>[2x]MAHHHHHHVDDDDKMNSDDNADGLIFSPLPQNKNTVVRHYSNEQEMPNLSQMAQRTIDFPTQIVRVSGNLTGLELSCDDVENEIDQVFSKKISPNLFTYNTYVSCGYDVNDPEQHATNFSIQSYFDPLTDNAVDYLKSYLKEYNGYNLFNTTTLQIENAKGIIVSMNLNAGL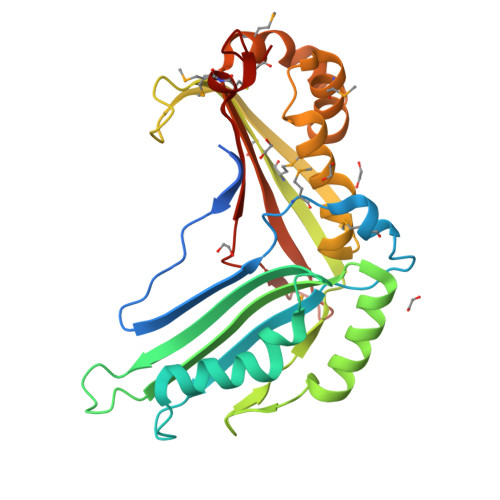KSNPDKTPFTLYRQDRNNFYFKSNFDVRKELISDIYQRFYSNDPDMILPFFDKWIFSYAGSVYYSILMASNYLELQPERIFVMENEGDIFVSDLRYYFANLCMKRNPNKHCL>[2x]GSHMA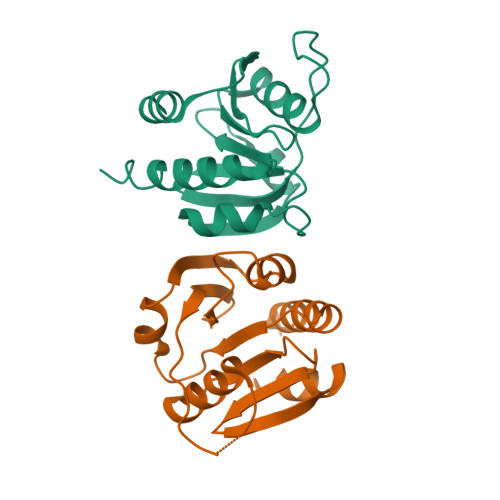SFFSRSGTPVEEAQQKTIEAITKAINYMAKRRIGALLTIERDTGMGDYIETGIPLNAKVSSELLINIFIPNTPLHDGAVIMKNNEIAAAACYLPLSESPFISKELGTRHRAAVGISEVTDSLTIIVSEETGGVSVAKNGDLHRELTEEALKEMLEAEFKKNTRDTSSNRWYWRGKKNG>[2x]MTKWVLHVDLDQFLASVELRRRPDLRGQPVIVGGSGDPSEPRKVVTTASYEAREFGVHAGMPLRAAARRCP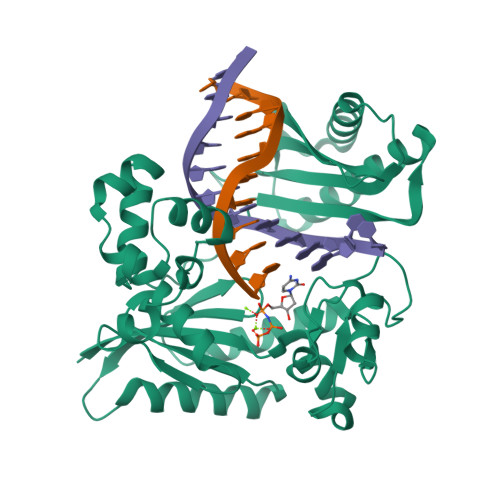DATFLPSDPAAYDEASEQVMGLLRDLGHPLEVWGWDEAYLGADLPDESDPVEVAERIRTVVAAETGLSCSVGISDNKQRAKVATGFAKPAGIYVLTEANWMTVMGDRPPDALWGVGPKTTKKLAAMGITTVADLAVTDPSVLTTAFGPSTGLWLLLLAKGGGDTEVSSEPWVPRSRSHVVTFPQDLTERREMDSAVRDLALQTLAEIVEQGRIVTRVAVTVRTSTFYTRTKIRKLPAPSTDAGQIVDTALAVLDQFELDRPVRLLGVRLELAMDDV(1S)-1-(4-chlorophenyl)-2-(1H-imidazol-1-yl)ethyl [4-(propan-2-yl)phenyl]carbamate | C21 H22 Cl N3 O2 | 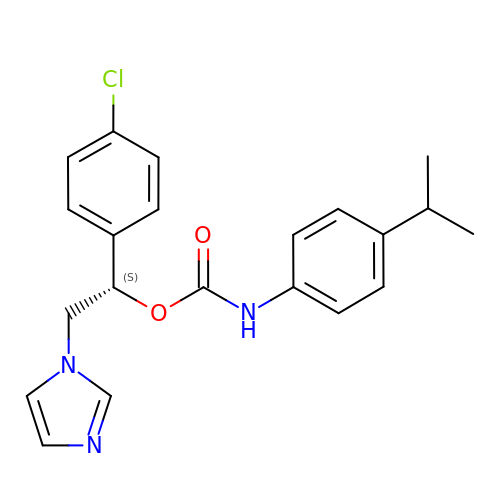JBMGTRUHKILUNG-HXUWFJFHSA-N>[2x]GSHMATPWSGYLDDVSAKFDTGVDNLQTQVTEALDKLAAKPSDPALLAAYQSKLSEYNLYRNAQSNTVKVFKD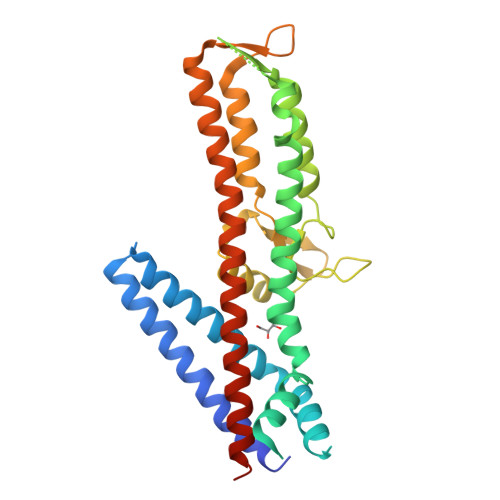IDAAIIQNFRGGSGGTTISDAEIWDMVSQNISAIGDSYLGVYENVVAVYTDFYQAFSDILSKMGGWLLPGKDGNTVKLDVTSLKNDLNSLVNKYNQINSNTVLFPAQSGSGVKVATEAEARQWLSELNLPNSCLKSYGSGYVVTVDLTPLQKMVQDIDGLGAPGKDSKLEMDNAKYQAWQSGFKAQEENMKTTLQTLTQKYSNANSLYDNLVKVLSSTISSSLETAKSFLQG> YEIIRTNVQEVLAEIVSPSTKNPNSENPAVKKRFRGIKNVVSRIISNDKKCRYDLIYNKYLSSSDTRKLKTMIDYSTKFNRVVEVVLIIMGKLLPLDAWGGTENKKVIQDRIVDFLRLGANERLHLDDVLSGIKLSKFKWLGVGNNISSQQDFQIRKRLLEGYINWVFISLVKNIVRAFWYVTESSNMDRSKLFYFTHSIWNELSSNWITKYAKGNLVQVVSPESKGQFTNGKIKLIPKRGGFRVICVPLKQSLYSFNNKRNFALKQKEKWDYIFYQKYTLSPVRQVLQLKLNALRKSDMGHRSSVNSTNEVADRILTFRNDLLKKNKTLPVLYMIKFDMKECYDRLNQNALKESIAGIFKEDNENTTYHVREYGTLDEFLKLKRVRTLIETEVQNFNIIMNSKDEAEAGSRSYGTKVDKVKTLSISKNKIIEVCHSQIEDATCLVKNKEGQYDLFKRKQGVFQGFSLSGIFCDILYSTMVSKEFKFLWEATEDNLLLRLVDDFIFITSNKD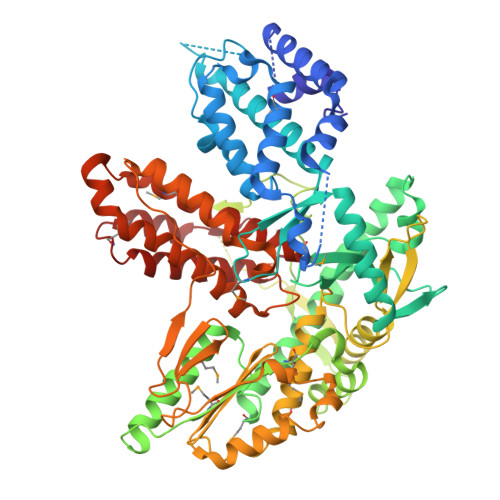TLKKVKDKISSNELQKYGAFVNHEKTVEINGEAGSSNKMTFVGLDINCLTLDVKKDSSQFSRPTCKFRSFKALFSNLKQFYCSNLSEFLLDFSSNSLETIRENVDAILKLTFEAIQTSFATISKQDSFERYRFMKFLHVIIETTIEKFARVNGSMEGVEYLLTCIKITITKSLAFMATKQEIIEWLYTLTIVD> PVFTQDVFVGSVEELSAAHTLVMKINATDADEPNTLNSKISYRIVSLEPAYPPVFYLNKDTGEIYTTSVTLDREEHSSYTLTVEARDGNGEVTDKPVKQAQVQIRILDVNDNIPVVENKVLEGMVEENQVNVEVTRIKVFDADEIGSDNWLANFTFASGNEGGYFHIETDAQTNEGIVTLIKEVDYEEMKNLDFSVIVA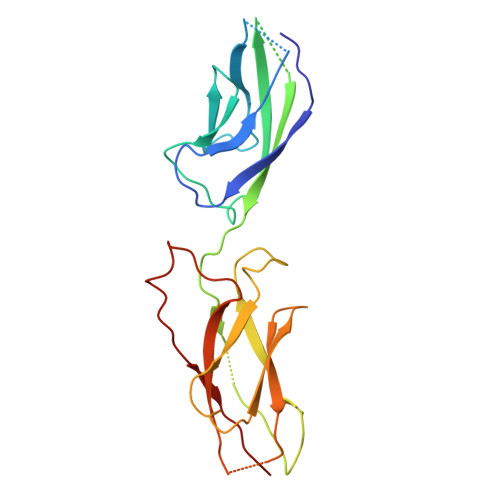NKAAFHKSIRSKYKPTPIPIKVKVK> MADEIDLYDDKGKKLAAGVPLQNISPLKNAAIKKIVNLTIRTGAVDLAGLEKKFATGAIAGRGMVIRGVNRNLPIVDKAKEIAKAVEDMLRVESGDDTNVELIAGGKRMMVQPPTARILSDYSVGLTASMGALTHAIIDVCNVSMWDAPYVHAGVWGMYPQNPDPGDGAVKMLVDIPMKNEGPGFTLRNIPVNHLAATVRKRAMQGAGLTMILEEAAQFEMGNCMGPHERGHLLDLAYEGLNANNLLYSLIKDNGQDGSLGDVIYAAVEKAKADGVIKSLKKMPSGFTVYDADDMQLWNAYACTAMLAGVCVNCASMRAGQPVPGNIMQACCLIERETGLPGPDFGMAQGA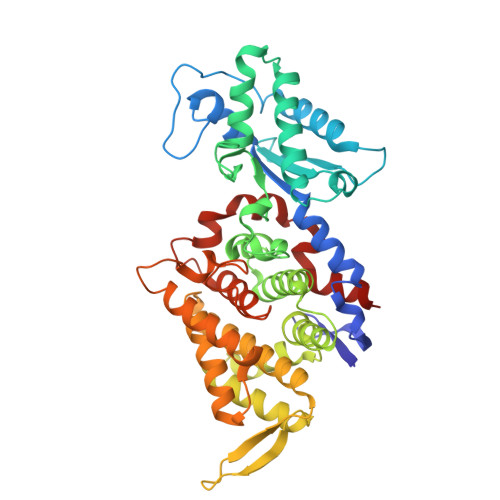SVSSSFFSHSIYGGGGPGVFYGNHIVTRHAKGQFIPCFCAAMCIDADTMYFSPARTSALYGEVLGAIPEFAEPMRAVAEAAK> GPDLPEGYEQRTTQQGQVYFLHTQTGVSTWHDPRVPRDLSNINCEELGPLPPGWEIRNTATGRVYFVDHNNRTTQFTDPRLSANLHLVLNRQNQLKDQQQQQVVSLCPDDTECLTVPRYKRDLVQKLKILR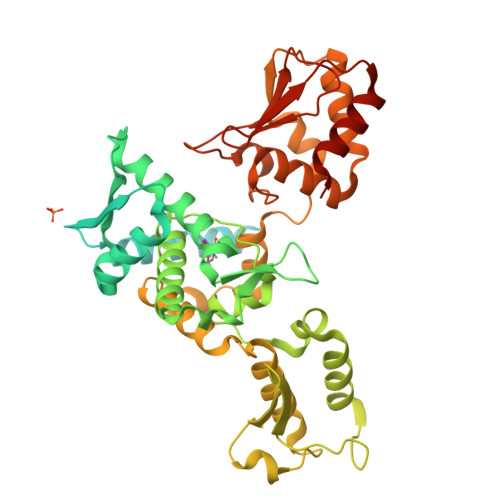QELSQQQPQAGHCRIEVSREEIFEESYRQVMKMRPKDLWKRLMIKFRGEEGLDYGGVAREWLYLLSHEMLNPYYGLFQYSRDDIYTLQINPDSAVNPEHLSYFHFVGRIMGMAVFHGHYIDGGFTLPFYKQLLGKSITLDDMELVDPDLHNSLVWILENDITGVLDHTFCVEHNAYGEIIQHELKPNGKSIPVNEENKKEYVRLYVNWRFLRGIEAQFLALQKGFNEVIPQHLLKTFDEKELELIICGLGKIDVNDWKVNTRLKHCTPDSNIVKWFWKAVEFFDEERRARLLQFVTGSSRVPLQGFKALQGAAGPRLFTIHQIDACTNNLPKAHTCFNRIDIPPYESYEKLYEKLLTAIEETCGFAVE>MGHHHHHHHHHHSSGHIEGRHMMATNLRGVMAALLTPFDQQQALDKASLRRLVQFNIQQGIDGLYVGGSTGEAFVQSLSEREQVLEIVAEEAKGKIKLIAHVGCVSTAESQQLAASAKRYGFDAVSAVTPFYYPFSFEE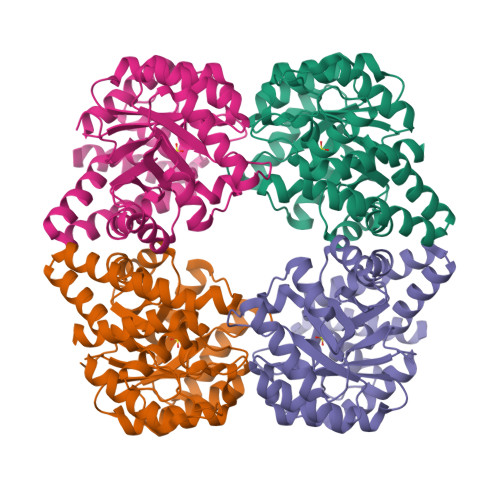HCDHYRAIIDSADGLPMVVYNIPALSGVKLTLDQINTLVTLPGVGALKQTSGDLYQMEQIRREHPDLVLYNGYDEIFASGLLAGADGGIGSTYNIMGWRYQGIVKALKEGDIQTAQKLQTECNKVIDLLIKTGIFRGLKTVLHYMDVVSVPLCRKPFGPVDEKYLPELKALAQQLMQERG[4x]>[4x]HHHHHHSSGLVPRGSHMASMSKVGINGFGRIGRLVLRRLLEVKSNIDVVAINDLTSPKILAYLLKHDSNYGPFPWSVDFTEDSLIVDGKSIAVYAEKEAKNIPWKAKGAEIIVECTGFYTSAEKSQAHLDAGAKKVLISAPAGEMKTIVYNVNDDTLDGNDTIVSVASCTTNCLAPMAKALHDSFGIE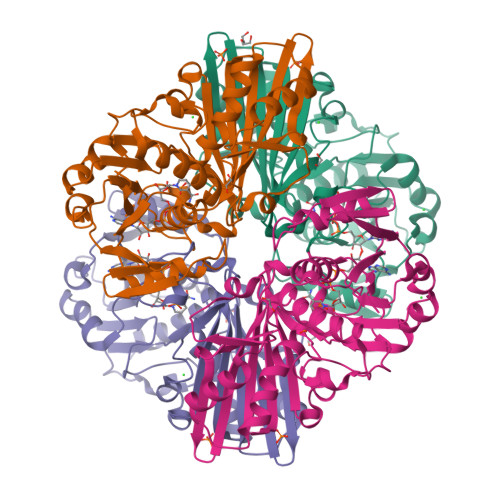VGTMTTIHAYTGTQSLVDGPRGKDLRASRAAAENIIPHTTGAAKAIGLVIPELSGKLKGHAQRVPVKTGSVTELVSILGKKVTAEEVNNALKQATTNNESFGYTDEEIVSSDIIGSHFGSVFDATQTEITAVGDLQLVKTVAWYDNEYGFVTQLIRTLEKFAKL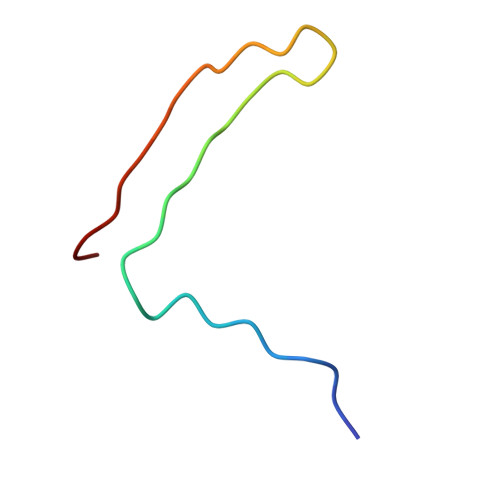> MAPEEIIMDRPFLFVVRHNPTGTVLFMGQVMEP>[2x]KSDIEIAQSVKLQDIREIAAKLGLTEDDIDLYGKYKAKVDYNLLNNCNGKKAKLILTTAITPTPAGEGKTTTTIGAADALTRLGKKTIVALREPSLGPVFGIKGGAAGGGYAQVVPMEDINLHFTGDIHAITAANNLLAAMVDNHIFQGNQLNIDTRRVVWRRAVDINDRQLRFVIDGLGGKANGVPREDGFDITVASEVMAIFCLANDIMDLKERLAKIVVAYDREGKPVTAGDLKAQGAMAALLKDALKPNLVQTLEGTPAFVHGGPFANIAHGCNSVIATKMAMHLADYVVTEAGFGADLGAEKFIDIKCRLAGLKPDAVIIVATVRALKYNGGLAKADLEKEDLNALAKGIPNL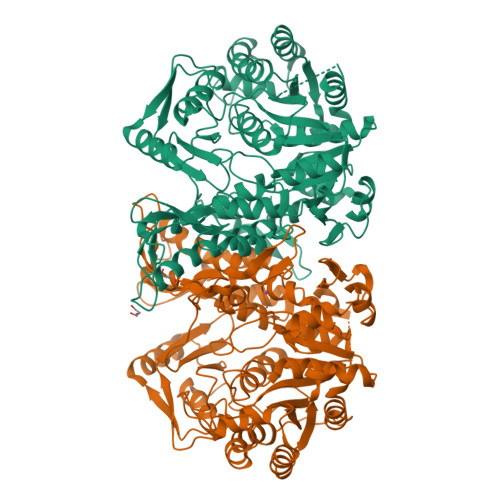LKHVENITQVFKLPAVVAINRFPQDTEAELKLVEDRCNELGVNVALSEVWAKGGEGGIALAEELIRLTEDNKASNKGLAYVYELDMPIEEKIRAISQKIYGADDVMFTDKALKEIANLEKLGFGKMPVCIAKTQYSLTDDPKKLGRPSGFNITVRDVSVSAGAGFIVAVTGDIMKMPGLPKVPAAEKIDVDEKGVISGLF>GIQPEKSVVFVAIDLEAYELDQSIITEVGLAILDTAEITNVAPGEGSKNWFDFIKARHIRVKEFSWAQNSRHVQGRAEYFDFGESEFIEVAKIASVLKETIEGESSIGGEGAKRPVVLVFHDQSQDLKYIRMLGYDVASADNILEVVDTREMYQYLSRSNNASKLSNVCGYLDIPWKNMHNAGNDAVYTLQAMMGLAIDMRQKSLERAAAKASKANTSNDGYVT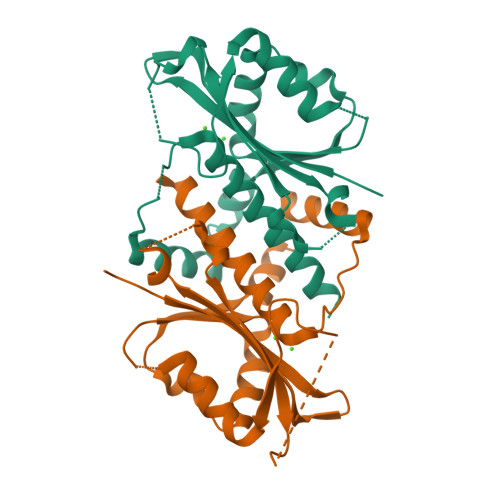YSEFTATKEDVDEGWI[2x]>MMFNFANFYQLIAQDTRLQPWLNVLPQQLTDWQNAEHGDFPRWLKALNKIPEGAPDQIDIKHSVTISNDTPFHQGELKKLESLLRTFHPWRKGPYTVHGIHIDTEWRSDWKWDRVLPHISPLKNRSVLDVGCGNGYHMW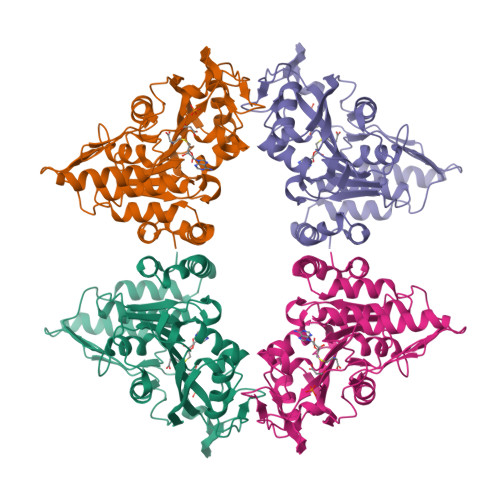RMLGEGARLCVGIDPSHLFLIQFEAIRKLMGGDQRAHLLPLGIEQLPKLEAFDTVFSMGVLYHRRSPLDHLIQLKDQLVSGGELILETLVIEGDETAVLVPKERYAQMRNVYFFPSARALKVWLELVGFEDVRIVDENVTSVDEQRTTNWMTHNSLPDYLDQNDPSKTVEGYPAPRRAILVAKKPGHHHHHHG[2x]>[4x]GAMDMKTLTTISGHSKDNLALLKCLQGETKEKEFEISNVLPNHKMKEKLFRENKLKIDIDIEKDIFNYSRKNIQKIEFMPVNRLISQSEIDGIIGTLKEVLPTGQFTSGPFSKKLEEVIGDYLNKKYVIATSSGTDALMVSLLSIGIQPGDEVIMPANSFAATENAVLAIGAKPVFVDIDHKSYCIDPLKIEEAITQKTKCILPVHLYGKQCDMKRIRE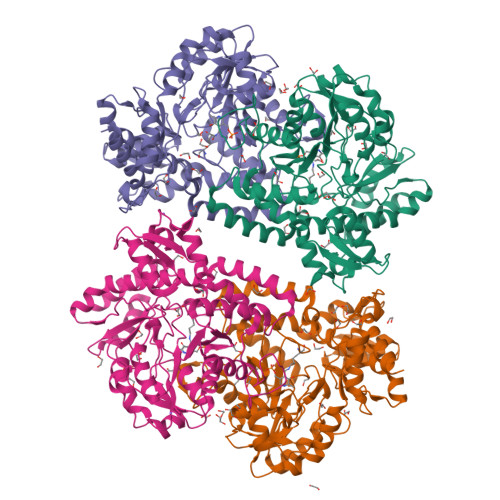IADVYQLRIIEDACQAIGSSNLGEYGDIIILSFNPYKNFGVCGKAGAIVTNNENLAIRCNQYSYHGFEVDKKNKKVLDFGFNSKIDNLQAAIGLERIKFLSYNNLKRVFLAQRYIRNLKELEDRELIKLPRMTEDNVWHLFPIRIINGRRDEVKNKLYQLYNIETDIYYPVLSHKHNTKLVKKNYMQDTLLNTEQVHKEILHLPLHPNMLLEEQNFVLEGLINVNK> MTHQTHTIAESNNFIVLDKYIKAEPTGDSYQSESDLERELIQDLRNQGYEFISVKSQSAMLANVREQLQNLNGVVFNDSEWRRFTEQYLDNPSDGILDKTRKIHIDYICDFIFDDERLENIYLIDKKNLMRNKVQIIQQFEQAGSHANRYDVTILVNGLPLVQIELKKRGVAIREAFNQIHRYSKESFNSENSLFKYLQLFVISNGTDTRYFANTTKRDKNSFDFTMNWAKSDNTLIKDLKDFTATCFQKHTLLNVLVNYSVFDSSQTLLVMRPYQIAATERILWKIKSSFTAKNWSKPESGGYIWHTTGSGKTLTSFKAARLATELDFIDKVFFVVDRKDLDYQTMKEYQRFSPDSVNGSENTAGLKRNLDKDDNKIIVTTIQKLNNLMKAESDLPVYNQQVVFIFDECHRSQFGEAQKNLKKKFKRYYQFGFTGTPIFPENALGSETTASVFGRELHSYVITDAIRDEKVLKFKVDYNDVRPQFKSLETETDEKKLSAAENQQAFLHPMRIQEITQYILNNFRQKTHRTFPGSKGFNAMLAVSSVDAAKAYYATFKRLQEEAANKSATYKPLRIATIFSFAANE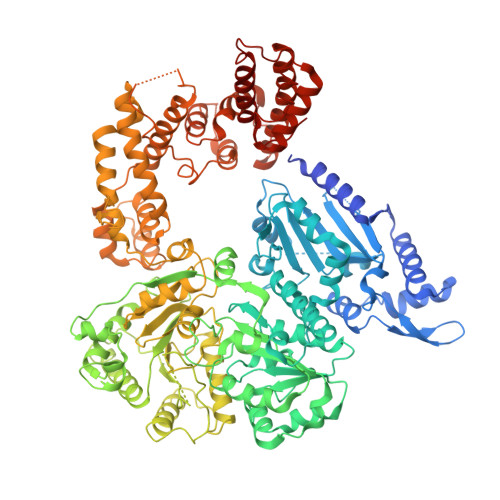EQNAIGEISDETFDTSAMDSSAKEFLDAAIREYNSHFKTNFSTDSNGFQNYYRDLAQRVKNQDIDLLIVVGMFLTGFDAPTLNTLFVDKNLRYHGLMQAFSRTNRIYDATKTFGNIVTFRDLERSTIDAITLFGDKNTKNVVLEKSYTEYMEGFTDAATGEAKRGFMTVVSELEQRFPDPTSIESEKEKKDFVKLFGEYLRAENILQNYDEFATLKALQQIDLSDPVAVEKFKAEHYVDDEKFAELQTIRLPADRKIQDYRSAYNDIRDWQRREKEAEKKEKSTTDWDDVVFEVDLLKSQEINLDYILGLIFEHNRQNKGKGEMIEEVKRLIRSSLGNRAKEGLVVDFIQQTNLDDLPDKASIIDAFFTFAQREQQREAEALIKEENLNEDAAKRYIRTSLKREYATENGTELNETLPKLSPLNPQYKTKKQAVFQKIVSFIEKFKGVGGKI> MSQRIIQPSASDQQFPGKSDGYEYTVGPKQAITSEASTTYIPSRIYSESLLFKRQEASLSAMAFLFQEMISQLHRTCKTAGDFETKLSDYGHNIGIRLLELLNFRASVSPSSLPRASAFLSQNESSSKLSNASNSP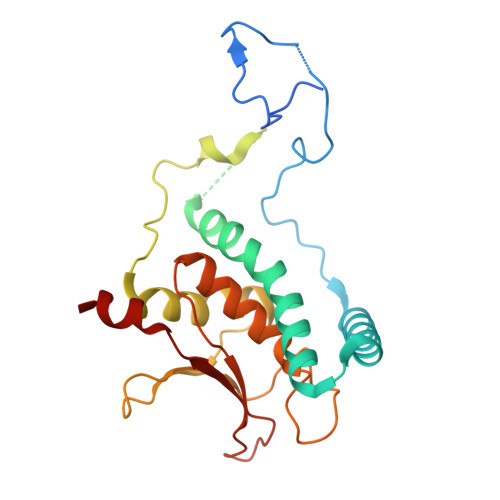GMLANSSTATSASANERLQEKQTESLSNYITKMRRRDLKILDILQFIHGTLWSYLFNHVSDDLVKSSERDNEYMIVDNFPTLTQFIPGENVSCEYFVCGIIKGFLFNAGFPCGVTAHRMPQGGHSQRTVYLIQFDRQVLDREGLRFG>[6x]MGHHHHHHHHHHSSGHIEGRHMMRA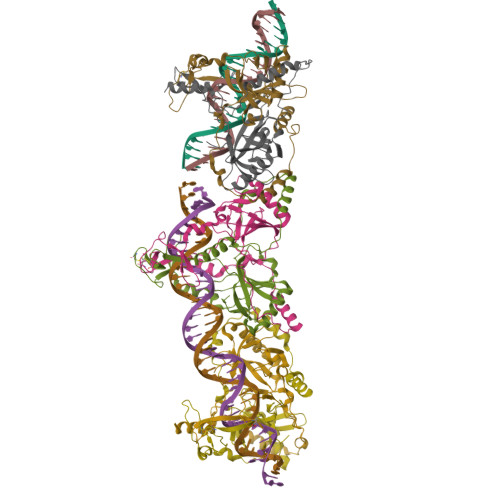IWTGSIAFGLVNVPVKVYSATADHDIRFHQVHAKDNGRIRYKRVCEACGEVVDYRDLARAYESGDGQMVAITDDDIASLPEERSREIEVLEFVPAADVDPMMFDRSYFLEPDSKSSKSYVLLAKTLAETDRMAIVHFTLRNKTRLAALRVKDFGKREVMMVHTLLWPDEIRDPDFPVLDQKVEIKPAELKMAGQVVDSMADDFNPDRYHDTYQEQLQELIDTKLEGGQAFTAEDQPRLLDEPEDVSDLLAKLEASVKARSKANSNVPTPP>HMMENINIVIKDVGYFQDKPQFLNSKSVRQWKHGTKVKLTKHNSHWYTGVVKDGNKSVRGYIYHSMAKVTSKNSDGSVNATINAHAFCWDNKKLNGGDFINLKRGFKGIT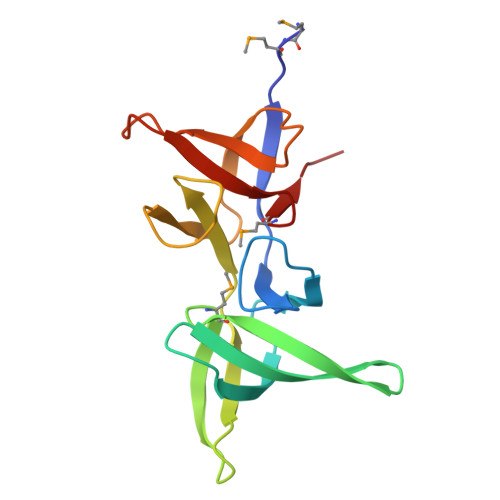HPASDGFYPLYFASRKKTFYIPRYMFDIKK[12x]>[2x]AFLGDGGDVSFSTRGTQNWTVERLLQAHRQLEERGYVFVGYHGTFLEAAQSIVFGGVRARSQDLDAIWRGFYI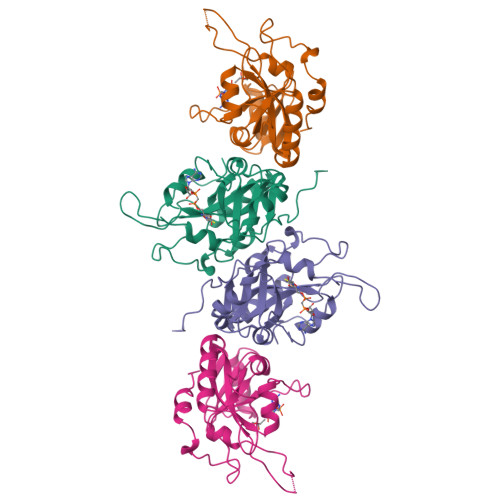AGDPALAYGYAQDQEPDARGRIRNGALLRVYVPRSSLPGFYRTSLTLAAPEAAGEVERLIGHPLPLRLDAITGPEEEGGRLETILGWPLAERTVVIPSAIPTDPRNVGGDLDPSSIPDKEQAISALPDYASQPGKPPR> MASETTPEDWKALAADVRSEFQWAWQGYVAKAWGKDEIN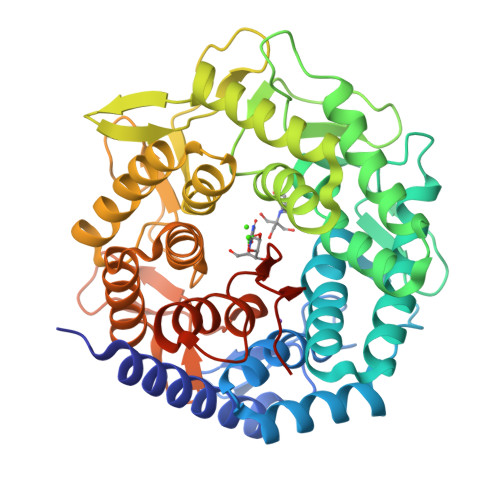PVSGTSRSFFIEGHDLGLSLVEALDTLWIMGLDAEFQAGVDWVKANLSFDVDGNAQVFETNIRLVGGLLSAHLASGDPVLLAKARDLADRLAKAFEASPHGLPWRYVNLRTGAVSDPETNLAEIGTYLSEFGVLSQLTGERKYFDMAKRAMRHTLDRRSKIGLMAANIHAMTGAFTSRNASIDVYADSFYEYLWDAWALFGDEDCKRWAVECVDAQLAHQAKRYDGRLWFPMVDFETGAVTGTAQSELAAYYAGLLGQVGRKAQGDDYLASFTYLQATFGVIPESIDVTTGQPRRKHTGLRPEYPDACLNLWLIDRDPRYRRLAAIHYREMKATSRAAFGYTALKDITTRPMTQDDNCPGYWWSEQMKYYYLLFSDTPRIDYGQLQLSTEANVLRGFRKVLEHHHHHH> GPHMLESRVSYDIEHLLYYSMSPHSWTLP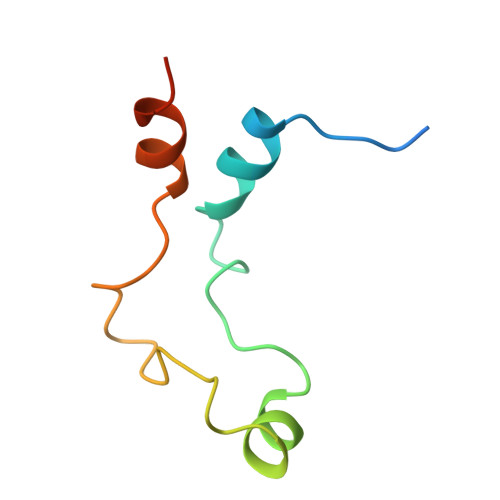TDWQKMQETAPSILRNKDLQDESQRFDGDKYLASIKTAAKR> APDTSVSNKQNFSTDVIYQIFTDRFSDGNPANNPTGAAFD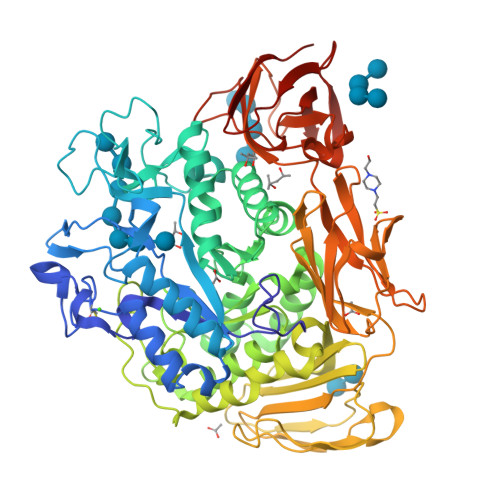GTCTNLRLYCGGDWQGIINKINDGYLTGMGVTAIWISQPVENIYSIINYSGVNNTAYHGYWARDFKKTNPAYGTIADFQNLIAAAHAKNIKVIINFAPNHTSPASSDQPSFAENGRLYDNGTLLGGYTNDTQNLFHHNGGTDFSTTENGIYKNLYDLADLNHNNSTVDVYLKDAIKMWLDLGIDGIRMDAVKHMPFGWQKSFMAAVNNYKPVFTFGEWFLGVNEVSPENHKFANESGMSLLDFRFAQKVRQVFRDNTDNMYGLKAMLEGSAADYAQVDDQVTFIDNHDMERFHASNANRRKLEQALAFTLTSRGVPAIYYGTEQYMSGGTDPDNRARIPSFSTSTTAYQVIQKLAPLRKSNPAIAYGSTQERWINNDVLIYERKFGSNVAVVAVNRNLNAPASISGLVTSLPQGSYNDVLGGLLNGNTLSVGSGGAASNFTLAAGGTAVWQYTAATATPTIGHVGPMMAKPGVTITIDGRGFGSSKGTVYFGTTAVSGADITSWEDTQIKVKIPAVAGGNYNIKVANAAGTASNVYDNFEVLSGDQVSVRFVVNNATTALGQNVYLTGSVSELGNWDPAKAIGPMYNQVVYQYPNWYYDVSVPAGKTIEFKFLKKQGSTVTWEGGSNHTFTAPSSGTATINVNWQP(5Z,8Z,11Z,14Z)-N-(2-hydroxyethyl)icosa-5,8,11,14-tetraenamide | C22 H37 N O2 | 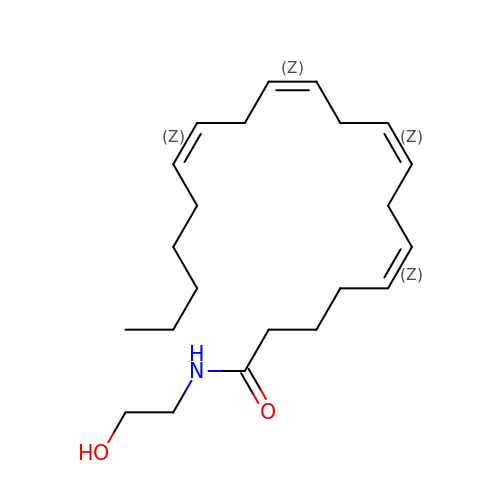LGEQQWMQCRIYKG-DOFZRALJSA-N> MHHHHHHSSGRENLYFQGMRRVVRQSKFRHVFGQAVKNDQCYDDIRVSRVTWDSSFCAV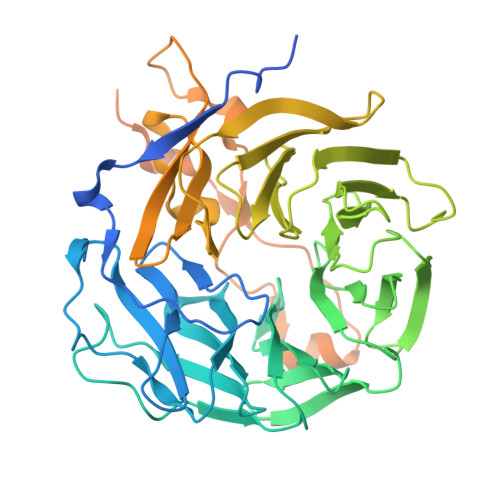NPRFVAIIIEASGGGAFLVLPLHKTGRIDKSYPTVCGHTGPVLDIDWCPHNDQVIASGSEDCTVMVWQIPENGLTLSLTEPVVILEGHSKRVGIVAWHPTARNVLLSAGCDNAIIIWNVGTGEALINLDDMHSDMIYNVSWNRNGSLICTASKDKKVRVIDPRKQEIVAEKEKAHEGARPMRAIFLADGNVFTTGFSRMSERQLALWNPKNMQEPIALHEMDTSNGVLLPFYDPDTSIIYLCGKGDSSIRYFEITDESPYVHYLNTFSSKEPQRGMGYMPKRGLDVNKCEIARFFKLHERKCEPIIMTVPRKSDLFQDDLYPDTAGPEAALEAEEWFEGKNADPILISLKHGYIPGKNRDLKVVKKNILDSKPTANKKCDLISIPKKTTDTASVQNEAKLDEILKEIKSIKDTICNQDERISKLEQQMAKIAA The capsid also protects the genome enroute to the nucleus for uncoating and replication. This study determines the capsid structures of TuV and CuV using cryo-electron microscopy and image reconstruction (cryo-EM) at ~2.9 Å resolution and compares them to the recently determined structure of BuV and other protoparvoviruses toward functional annotation. The VP ORF encodes two overlapping structural proteins, VP1 and VP2, sixty copies of which assemble the T = 1 icosahedral capsid in an approximate 1:10 ratio, respectively. The individual VPs contain an eight-stranded (βB to βI) anti-parallel β-barrel motif, with the βBIDG sheet forming the interior surface of the capsid. The virus capsid plays a central role in the infection by the protoparvoviruses as it mediates the attachment of the virus to specific receptors on target cells.

In 2016, CuV was found in human fecal samples and cutaneous T-cell lymphomas (CTCL). In the CuV capsid, the depression at the 2-fold (blue to cyan colors, corresponding to a distance of <110 Å from the center of the capsid) is broad, continuous, and has a slight diagonal tilt relative to the icosahedral 2-fold axes. While CuV’s VR1 is extended compared to MVMp due to a five amino acid insertion, VR3 is one amino acid shorter and adopts a different conformation. The absence of this loop separates the 3-fold protrusions in the CuV capsid while the loop merges the 3-fold protrusions in MVMp as well as protoparvoviruses CPV, FPV, PPV, H1-PV, and LuIII, which all share this loop. In contrast to TuV, the two highest signals showed glycans with α2-6-linked SIA in a 6’SLN (N-acetylneuraminic acid-α2-6-galactose-β1-4-N-acetyl- glucosamine) context. In contrast, CuV possesses a lysine in the same position (K377), which is similar to the CPV variant (R377K) unable to bind SIA. Thus, while TuV might bind SIA in a similar way to MVM or CPV, CuV’s SIA binding is likely different due to sequence and structural variability in the capsid’s surface loops.

>[60x]GSGVGHSTGDYNNRTEFIYHGDEVTIICHSTRLVHINMSDREDYIIYETDRGPLFPTTQDLQGRDTLNDSYHAKVETPWKLLHANSWGCWFSPADFQQMITTCRDIAPIQMHQKIENIVIKTVSKTGTGETETTNYNNDLTALLQIAQDNSNLLPWAADNFYIDSVGYVPWRACKLPTYCYHVDTWNTIDINQADTPNQWREIKKGIQWDNIQFTPLETMINIDLLRTGDAWQSGNYTFHTKPTNLAYHWQSQRHTGSCHPTVAPLVERGQGTNIQSVNCWQWGDRNNPSSASTRVSNIHIGYSFPEWQIHYSTGGPVINPGSAFSQAPWGSTTEGTRLTQGASEKAIYDWSHGDDQPGARETWWQNNQHATGQTDWAPKNAHTSELNNNVPAATHFWKNSYHNTFSPFTAVDDHGPQYPWGAIWGKYPDTTHKPMMSAHAPFLLHGPPGQLFVKLAPNYTDTLDNGGITHPRIVTYGTFWWSGKLVFKGKLRTPRQWNTYNLPSLDKRETMKNTVPNEVGHFELPYMPGRCLPNYTL>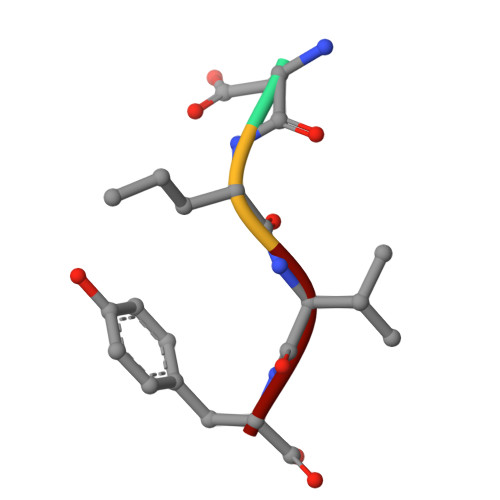 DRVY> MRLFGYARVSTSQQSLDIQVRALKDAGVKANRIFTDKASGSSSDRKGLDLLRMKVEEGDVILVKKLDRLGRDTADMIQLIKEFDAQGVSIRFIDDGISTDGEMGKMVVTILSAVAQAERQRILERTNEGRQEAMA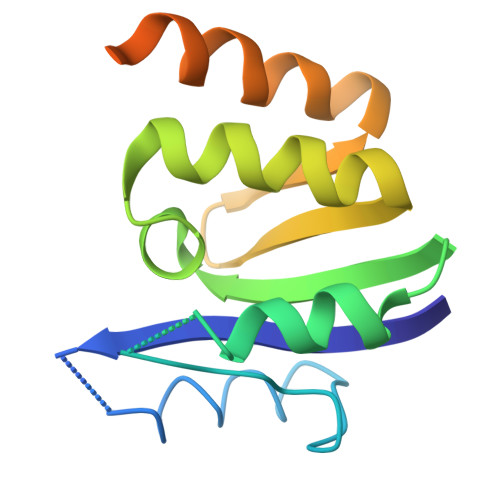KGVVF> MGSSHHHHHHSSGLVPRGSQSTSLYKKAGLMNIIIATTKSWNIKNAQKFKKENESKYNTTIITNKDELTFEKVKLINPEYILFPHW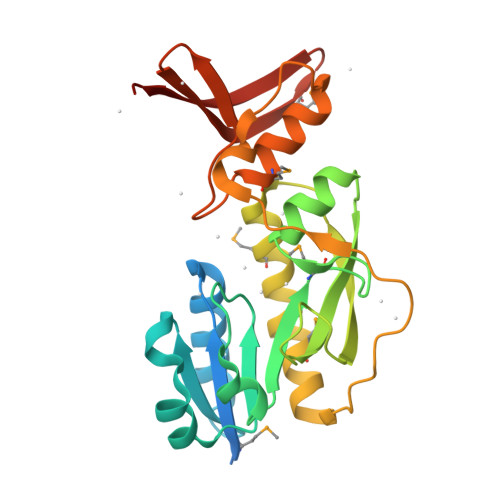SWIIPKEIFENFTCVVFHMTDLPFGRGGSPLQNLIERGIKKTKISAIKVDGGIDTGDIFFKRDLDLYGTAEEIFMRASKIIFNDMIPELLTKRPVPQKQEGEATVFQRRKPEQSEISPDFDLEKIYDYIRMLDGEGYPRAFIKYGKYRLEFSRASMKNGKIIADVEIIEGDENE>[8x]ASQTITVGPWG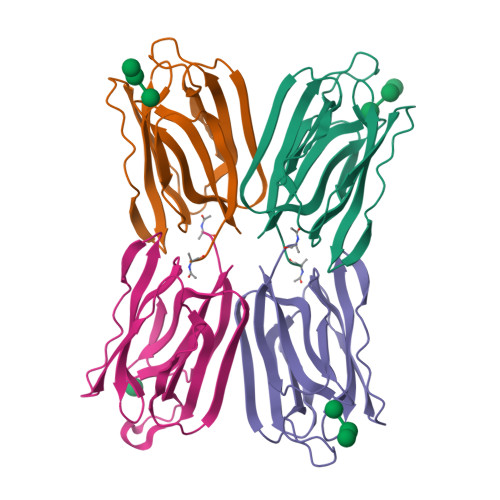GPGGNGWDDGSYTGIRQIELSYKEAIGSFSVIYDLNGDPFSGPKHTSKLPYKNVKIELKFPDEFLESVSGYTGPFSALATPTPVVRSLTFKTNKGRTFGPYGDEEGTYFNLPIENGLIVGFKGRTGDLLDAIGIHMSL>[2x]AEPVYPDQLRLFSLGQGVCGDKYRPVNREEAQSVKSNIVGMMGQWQISGLANGWVIMGPGYNGEIKPGTASNTWCYP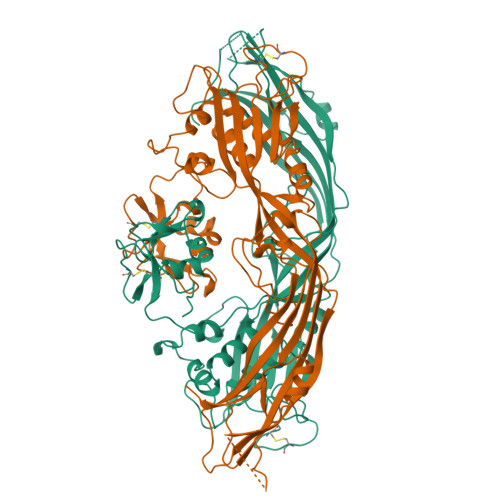TNPVTGEIPTLSALDIPDGDEVDVQWRLVHDSANFIKPTSYLAHYLGYAWVGGNHSQYVGEDMDVTRDGDGWVIRGNNDGGCDGYRCGDKTAIKVSNFAYNLDPDSFKHGDVTQSDRQLVKTVVGWAVNDSDTPQSGYDVTLRYDTATNWSKTNTYGLSEKVTTKNKFKWPLVGETELSIEIAANQSWASQNGGSTTTSLSQSVRPTVPARSKIPVKIELYKADISYPYEFKADVSYDLTLSGFLRWGGNAWYTHPDNRPNWNHTFVIGPYKDKASSIRYQWDKRYIPGEVKWWDWNWTIQQNGLSTMQNNLARVLRPVRAGITGDFSAESQFAGNIEIGAPVPLAADSKVRRARSVDGAGQGLRLEIPLDAQELSGLGFNNVSLSVTPAANQ>MRKTRYIQEGTVSLALLPALVVSAGIPLHNRKAQINTPCDASHYAAAVADNAVSAFEQALGRAQDATVAANKLHLLASKLAGAQKAATTILAAAAGAAAADAIQKIAAATPNFAKGFAALNEIKGGQIIVDEMLKSKIEDAATVAAASSTSGATIVKIKPKLQPATKRACHDEQGKPTKTQDKAVEVAGDITLTLFSLKAETPGTTTDQKLTLCGHGSPSQDPATASCQNSQANLGIKGGSFIVKHQMQTTRTTTGATASYSAIASEDTVPNGDTITAQLTEIAKLENAVQALQNVHESAEAKSLAGKSDIKEVVARALAGETASYADTKIQKQVDGFLEAVFGKDASTVTG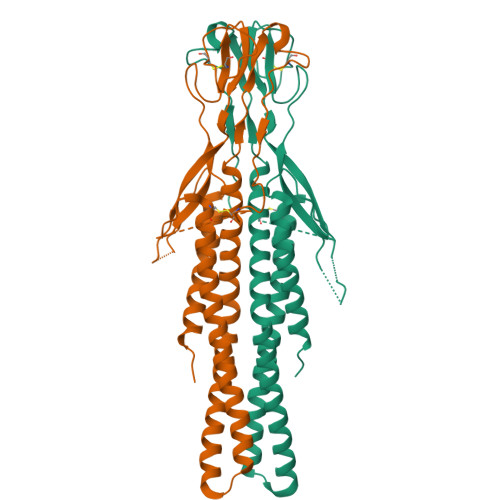VIVKELKDLIPPKVAFSGAGNTKLEEITDPNQIADATTYYTVRSYIADQEEKNKSSTSPSCTTKTEKAKEPAKTTDECKKHTTNDACKKEKGCDFDEKKDPKCFPKVETEKKDEKSFSSNLRVSVPQVFAAFAALLF[2x]>[2x]GMARKRLIIEMGMGIDQHGQE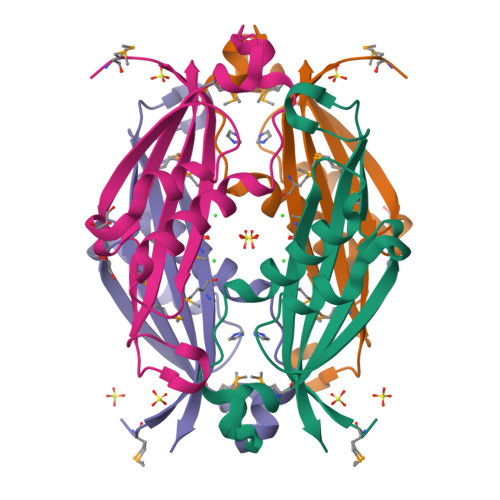PTIAASRAVRNAIAHNALPGVWEVAGLSHPNEMIIEVQVAVPYPEQVREEEVLAVLPFGRKTLTVESGGMIVQGRAIPELNDKNDEMLIAIAAVTVLIENE>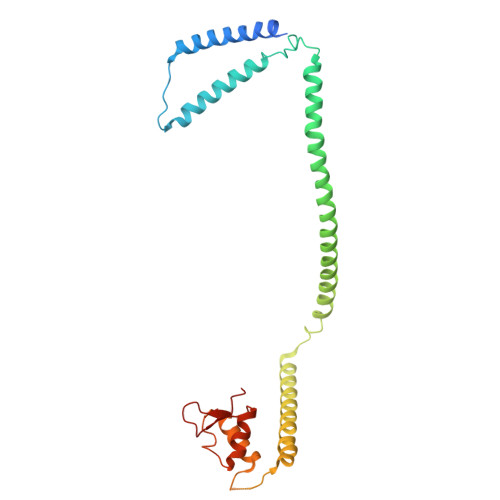 MNQEDLDPDSTTDVGDVTNTEEELIRECEEMWKDMEECQNKLSLIGTETLTDSNAQLSLLIMQVKCLTAELSQWQKKTPETIPLTEDVLITLGKEEFQKLRQDLEMVLSTKESKNEKLKEDLEREQRWLDEQQQIMESLNVLHSELKNKVETFSESRIFNELKTKMLNIKEYKEKLLSTLGEFLEDHFPLPDRSVKKKKKNIQESSVNLITLHEMLEILINRLFDVPHDPYVKISDSFWPPYVELLLRNGIALRHPEDPTRIRLEAFHQ>QEFTIDFSTQQSYVSSLNSIRTAISTPLEHISQGATSVSVINHTPPGSYISVGIRGLDVYQAHFDHLRLIIEQNNLYVAGFVNTATNTFYRFSDFAHISLPGVTTISMTTDSSYTTLQRVAALERSGMQISRHSLVSSYLALMEFSGNTMTREASRAVLRFVTVTAQALRFRQIQREFRQALSETAPVYTMTPEDVDLTLNWGRISNVLPEYRGEDGVRVGRISFNNISAILGTVAVILNCHHQGARSVRAVNEESQPECQITGDRPVIKINNTLWESNTAAAFLNRKSQSLYTTGE[2x];>[10x]ADCAKGKIEFSKYNENDTFTVKV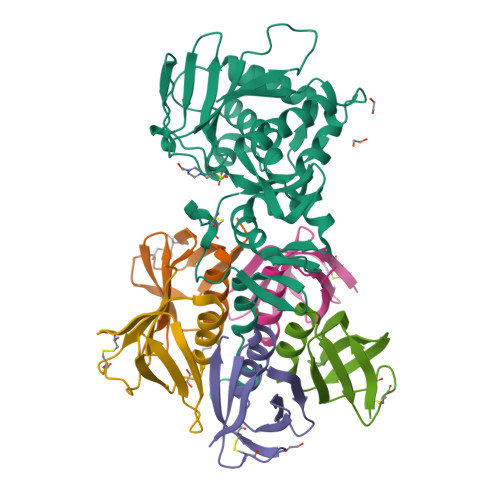AGKEYWTNRWNLQPLLQSAQLTGMTVTIKSSTCASGSGFAEVQFNND> DDDLVDAEGNLVENGGTYYLLPHIWAHGGGIETAKTGNEPCPLTVVRSPNEVSKGEPIRISSQFRSLFIPRGSLVALGFANPPSCAASPWWTVVDSPQGPAVKLSQQKLPEKDILVFKFEKVSHSNIHVYKLLYCQHDEEDVKCDQYIGIHRDRNGNRRLVVTEENPLELVLLKAKSETASSH;> IVGGYTCGANTVPYQVSLNSGYHFCGGSLINSQWVVSAAHCYKSGIQVRLGEDNINVVEGNEQFISASKSIVHPSYNSNTLNNDIMLIKLKSAASLNSRVASVSLPTSCASAGTQCLISGWGNTKSSGTSYPDVLKCLKAPILSDSSCKSAYPGQITSNMFCAGYLEGGKDSCQGDSGGPVVCAGKLQGIVSWGSGCAQKNKPGVYTKVCNYVSW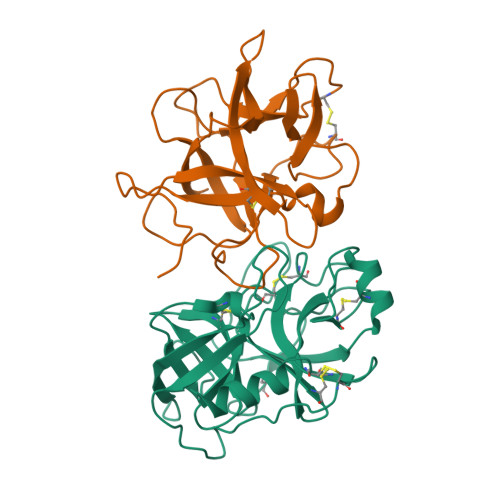IKQTIASN>[2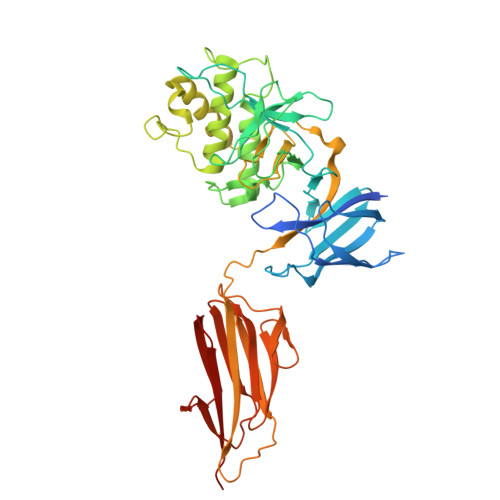x]MAHHHHHHSSGLEVLFQGPNQPQTTSVLIRKYAIGDYSKLLEGATLQLTGDNVNSFQARVFSSNDIGERIELSDGTYTLTELNSPAGYSIAEPITFKVEAGKVYTIIDGKQIENPNKEIVEPYSVEAYNDFEEFSVLTTQNYAKFYYAKNKNGSSQVVYAFNADLKSPPDSEDGGKTMTPDFTTGEVKYTHIAGRDLFKYTVKPRDTDPDTFLKHIKKVIEKGYREKGQAIEYSGLTETQLRAATQLAIYYFTDSAELDKDKLKDYHGFGDMNDSTLAVAKILVEYAQDSNPPQLTDLDFFIPNNNKYQSLIGTQWHPEDLVDIIRMEDKKEVIPVTHNLTLRKTVTGLAGDRTKDFHFEIELKNNKQELLSQTVKTDKTNLEFKDGKATINLKHGESLTLQGLPEGYSYLVKETDSEGYKVKVNSQEVANATVSKTGITSDETLAFENNKEPVVPT Host proteases, TMPRSS2 and CTSL/CTSB cleave the SARS-CoV-2 spike to play a crucial role in the two alternative pathways of viral entry and are characterized as promising pharmacological targets. The entry of SARS-CoV-2 depends on two distinctive pathways, cell surface entry and endosomal entry, where the transmembrane serine protease, TMPRSS2, and endosomal cysteine proteases cathepsin L/B (CTSL/CTSB) cleave the viral spike protein. The crystal structures of TMPRSS2 and CTSL/CTSB in complex with the potent inhibitors were determined to reveal their specific mode of interaction.

Nafamostat and camostat, two clinically available drugs used to treat pancreatitis, displayed excellent inhibitory potency with IC50 values of 0.40 nM and 9.00 nM, respectively. The crystal structures of TMPRSS2 in complex with nafamostat, camostat, and UK-371804, were determined to 2.6 Å, 2.4 Å and 2.6 Å, respectively. We use the structure of TMPRSS2 in complex with camostat as the representative to describe the overall structure of TMPRSS2. There are two polypeptides in the asymmetric unit with the root-mean-square deviation (r.m.s.d) of 1.44 Å over 378 Cα atoms, indicating the two protomers are similar. The ectodomain of TMPRSS2 can be traced in the electron density map except for several small loop regions (residues 109–112, 202–205, 229–230, and 250–255). The ester group in their common guanidinobenzoyl moiety then reacts with the catalytic serine of TMPRSS2 to form the acyl-enzyme intermediate and cleave off the “leaving group”. The guanidinobenzoyl group stays covalently linked to the catalytic serine and disables the protease activity. Our structures of TMPRSS2 in complex with nafamostat and camostat both capture the post-reaction state, leaving the identical remnant moiety in the catalytic site of the SP domain. Apart from the ester bond formed with γO of the catalytic serine, the guanidyl head of the guanidinobenzoyl moiety forms a salt bridge with Asp435, and is further anchored by hydrogen bonds with Ser436 and Gly464 in the S1 pocket.

>[2x]MGSKCSNSGIECDSSGTCINPSNWCDGVSHCPGGEDENRCVRLYGPNFILQVYSSQRKSWHPVCQDDWNENYGRAACRDMGYKNNFYSSQGIVDDSGSTSFMKLNTSAGNVDIYKKLYHSDACSSKAVVSLRCIACGVNLNDDDDK;>[2x]IVGGESALPGAWPWQVSLHVQNVHVCGGSIITPEWIVTAAHCVEKPLNNPWHWTAFAGILRQSFMFYGAGYQVEKVISHPNYDSKTKNNDIALMKLQKPLTFNDLVKPVCLPNPGMMLQPEQLCWISGWGATEEKGKTSEVLNAAKVLLIETQRCNSRYVYDNLITPAMICAGFLQGNVDSCQGDSGGPLVTSKNNIWWLIGDTSWGSGCAKAYRPGVYGNVMVFTDWIYRQMRADGEFVEHHHHHHHH1-(3,5-dihydro-2~{H}-1,4-benzothiazepin-4-yl)ethanone | C11 H13 N O S | 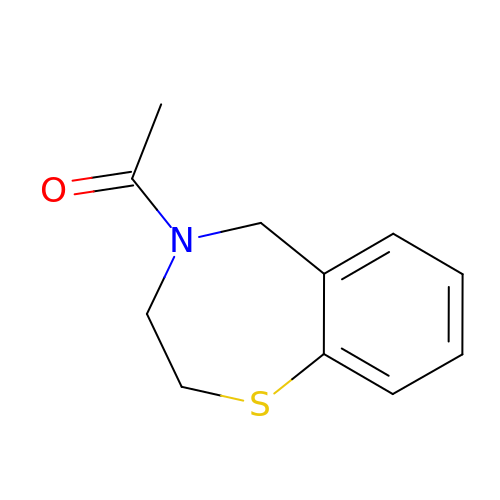UREQFTSPNGUYSJ-UHFFFAOYSA-N>QIQPKPGFCVKTNSSEGKVFINICHSPSIPPPADVTEDELLQMLEEDQAGFRIPMSLGEPHAELDAKGQGCTAYDVAVNSNFYLRMQNSDFLRELVVTIAREGLEDKYGLQLNPEWRMLKYRSFLGSISQQNI[2x];>[2x]SELDSDDEF

The R2TP complex is found in organisms from yeast to humans, and consists of the AAA+ ATPases Rvb1 and Rvb2 (human: RUVBL1 and RUVBL2), a TPR-containing protein, Tah1 (human: Spagh or RPAP3), and Pih1 (also known as NOP17 and Pih1D1, but referred to as Pih1 henceforth; Kakihara and Houry, 2012; Te et al., 2007). Pih1 is the multipoint scaffold of the R2TP complex, coupling the Rvb1-Rvb2 hetero-dodecamer, the Hsp90 chaperone machinery (via Tah1 in yeast or Spagh/RPAP3 in metazoa), and the TTT (Tel2-Tti1-Tti2) complex implicated in activation and stabilization of PIKKs (Hurov et al., 2010; Kakihara and Houry, 2012). The biological roles ascribed to the R2TP complex are directly associated with its ability to interact with the Hsp90 chaperone system and function as an Hsp90 cochaperone (Boulon et al., 2010; Izumi et al., 2012; Takai et al., 2010). Here we present crystal structures of Hsp90-Tah1-Pih1, Hsp90-Spagh/RPAP3, and Pih1-Tel2 complexes that together define key structural links within the R2TP core in yeast and in animals and reveal how R2TP connects the Hsp90 chaperone system to the TTT complex involved in PIKK activation.

Interaction with Tel2 involves the N-terminal segment of Pih1 (Horejsí et al., 2010), which contains a conserved region of unknown structure (henceforth, PIH domain). We determined the crystal structure of the mouse PIH domain1–200 with single-wavelength anomalous dispersion phasing of Tel2-peptide cocrystals (see below) grown with SeMet protein (see Experimental Procedures) and used this to phase the mPih47–179 apo and SELDpSDDEF peptide-bound structures, which were refined to 2.1 and 3.3 Å, respectively. We next obtained crystals of a complex of the PIH domain and the Ser 488-Ser 492-bis-phosphorylated Tel2 peptide. The phosphopeptide binds to an intensely basic patch in the high-resolution apo-structure formed by the loop connecting β strands 3 and 4; the faces of β strands 1, 2, and 5; and the coil segment C-terminal to β strand 5. Electron density is evident for the Tel2 peptide from residue 488 to 496, but side chains are only well defined for residues 489–495. The Tel2 phosphopeptide binds as a 310 helix stabilized by a backbone peptide hydrogen bond between Asp 491-C=O and Asp 494-NH and reinforced by a hydrogen bond between the side chain of Asp 491 and Asp 493-NH. The core of the PIH domain interaction with the Tel2 phosphopeptide is provided by interlinked hydrogen bonds between the side chains of Lys 57, Lys 64, and Lys 113 from Pih1, and the side chain phosphate and carboxyl groups of pSer 492, Asp 491, and Asp 493 from Tel2. This is reinforced by hydrogen bonds from the side chains of Asp 493 and Asp494 of Tel2 with the peptide NHs of Lys 166 and Ala 112 of Pih1, respectively. An additional hydrophobic interaction is provided by Tel2-Phe 496, which slots into a small crevice formed by the side chains of Ala 112, Arg 168, and Leu 171 of Pih1.> STSKDHVKSQIPRLSAINDLHKIWPTVEEHGAAIIESFLSLDIVRRLNEEVDPFVKIEPIPAAKTKDHPNHKLSTTTRLVNVLAPISKAYREDVLNSKVLHRICSDAFHVYGDYWVLMGAVMELAPSNPAQPLHRDMRFSHPIVEYLKPDAPATSINFLVALSPFTAENGATHVILGSHKWQNLSNVSMDATVRALMNPGDALLITDSTIHCGGAETTGTETRRLLTITMGISQLTPLESNLAVPRPVIESLTPLAQRLLGWASQRSAAPRDIGLLTIRGNSIEKTMNLKAEQPLHDDEAEPLCRETI

The non-heme FeII/α-ketoglutarate-dependent dioxygenase AsqJ from Aspergillus nidulans is an exceptional enzyme that activates dioxygen and stereoselectively catalyzes a C–C bond desaturation and epoxidation reaction. AsqJ converts its natural substrate, 4′-methoxycyclopeptin, to a quinolone alkaloid, 4′-methoxyviridicatin. The active site of AsqJ forms a funnel like reaction chamber, located at the interface between antiparallel β-strands. The substrate interacts with the active site metal, which is ligated by His-211, His-134, Asp-136, as well as by the C-2 keto group and C-1 carboxylate of α-ketoglutarate (αKG), and a crystallographic water molecule in an octahedral coordination sphere.

For comparison, we also studied the effect of the V72K, V72L, and F139I substitutions to increase the interaction between His-134 and the substrate from the opposite side. However, whereas the V72K and V72L mutants did not improve the π-stacking interactions, the F139I variant showed some minor increase in the dispersive interactions between His-134 and the surrogate. To this end, we cloned, expressed, and purified the V72I-, V72K-, and F139I-mutated AsqJ enzymes. The catalytic activities of these mutants were determined for the native substrate 1, cyclopeptine 1b, as well as for demethylcyclopeptine 1d and compared to the wild-type (wt) AsqJ by using a reverse-phase HPLC/MS-coupled activity assay, and X-ray crystallography. The wt and V72I-, V72K-, F139I-mutated AsqJ variants turned out to have similar turnover rates for the methylated substrates 1 and 1b, suggesting that these alterations do not lead to a significant decrease in the enzyme activity. In contrast, the F139I mutant only displays a minor increase in activity, whereas the turnover of V72K for 1d is similar to the wt enzyme as proposed by our MD simulations.>SRNVPFPYAETDVADLQARMTAGELDSTTLTQAYLQRIAALDRTGPRLRAVIELNPDALKEAAERDRERRDGRLRGPLHGIPLLLKDNINAAPMATSAGSLALQGFRPDDAYLVRRLRDAGAVVLGKTNLSEWANFRGNDSISGWSARGGQTRNPYRISHSPCGSSSGSAVAVAANLASVAIGTETDGSIVCPAAINGVVGLKPTVGLVSRDGIIPISFSQDTAGPMARSVADAAAVLTAIAGRDDADPATATMPGRAVYDYTARLDPQGLRGKRIGLLQTPLLKYRGMPPLIEQAATELRRAGAVVVPVELPNQGAWAEAERTLLLYEFKAGLERYFNTHRAPLRSLADLIAFNQAHSKQELGLFGQELLVEADATAGLADPAYIRARSDARRLAGPEGIDAALAAHQLDALVAPTTGVAWPIRSEGDDFPGESYSAAAVAGYPSLTVPMGQIDGLPVGLLFMGTAWSE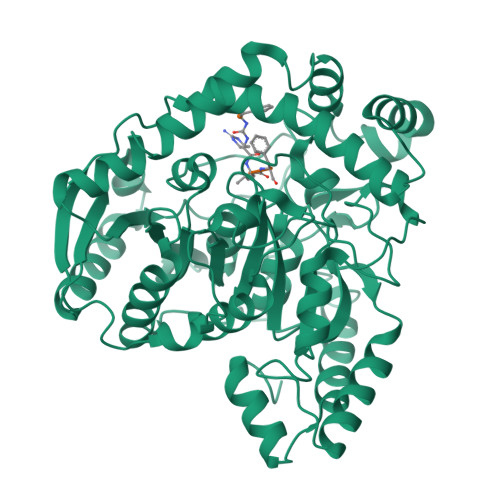PKLIEMAYAYEQRTRARRPPHFDTDALIDAGEP[2x]(4~{S})-6-azanyl-4-[3-(2-chlorophenyl)-5-(trifluoromethyl)phenyl]-3-methyl-4-propan-2-yl-2~{H}-pyrano[2,3-c]pyrazole-5-carbonitrile 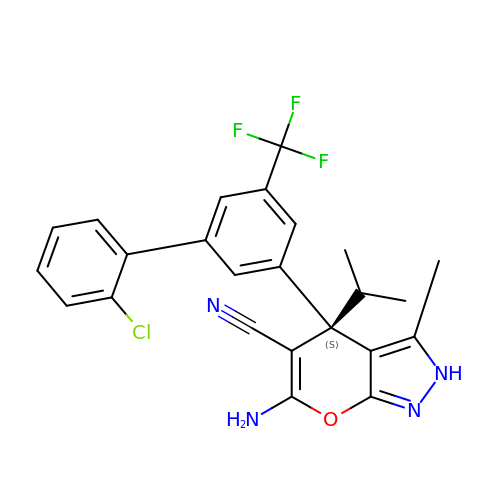| C24 H20 Cl F3 N4 O | MHJHVTMVGRIZDH-QHCPKHFHSA-N>MDEFEMIKRNTSEIISEEELREVLKKDEKSAYIGFEPSGKIHLGHYLQIKKMIDLQNAGFDIIILLADLHAYLNQKGELDEIRKIGDYNKKVFEAMGLKAKYVYGSEFQLDKDYTLNVYRLALKTTLKRARRSMELIAREDENPKVAEVIYPIMQVNDIHYLGVDVAVGGMEQRKIHMLARELLPKKVVCIHNPVLTGLDGEGKMSSSKGNFIAVDDSPEEIRAKIKKAYCPAGVVEGNPIMEIAKYFLEYPLTIKRPEKFGGDLTVNSYEELESLFKNKELH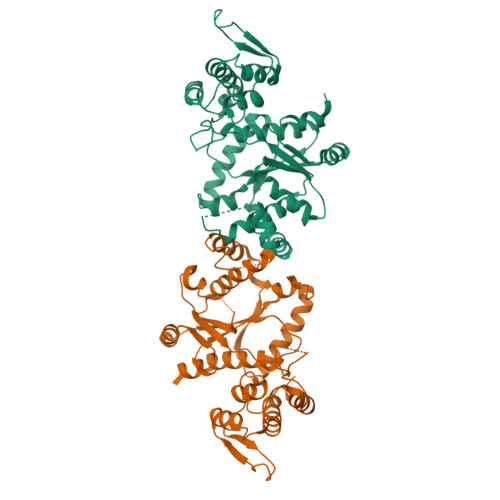PMDLKNAVAEELIKILEPIRKRL[2x]>[2x]MATERQAAIAKKRQTDKALNKKAALKNSQLSRKINQTTFSNNKNTDEQVTKALNLSHFVGSALVVKNDHVIYNRAFGYANKAKNQRNKVNSKYQILSIQKSMTAVGIMQLVQAGKVKLTDPISKYYPTLKHGR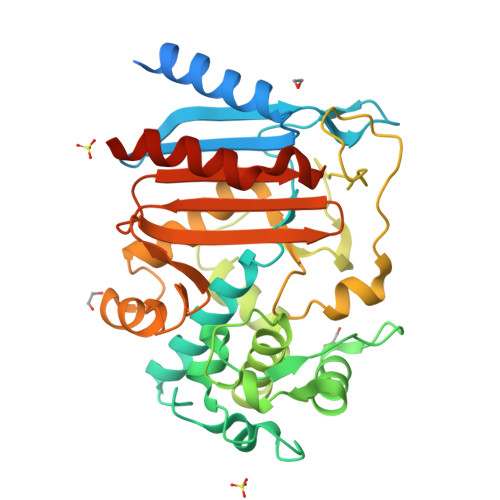QTTLRQMLDMTTGFRLKSGSKEFLPENQVIDFAAHNVFYYPDKNGIYNYSSVNFLLLAGIIRKVTGQSYQHFFTTHFIDKLNLNETGFLIHGQGQDATTGYRALADQTLPNYDQTMPESKSQMANELGTGQVYMSTADLFTVESAILKGQLLSKKNVAILHTRTATGEYGGGVYNMSNGIRSHGLGYGYESSIFLSPDGKTGVVLMSNYYRKAAGIQATANKIFTELMKGDIKLEHHHHHH>[2x]GSHGQYLLPEAKAQDSDKICVVINLDETLVHSSFKPVNNADFIIPVEIDGV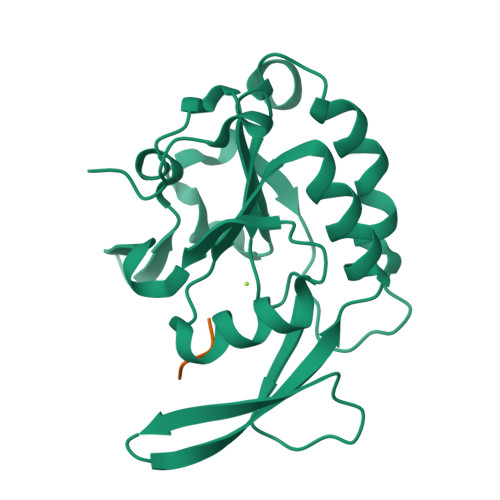VHQVYVLKRPHVDEFLQRMGELFECVLFTASLAKYADPVADLLDKWGAFRARLFRESCVFHRGNYVKDLSRLGRDLRRVLILDNSPASYVFHPDNAVPVASWFDNMSDTELHDLLPFFEQLSRVDDVYSVLRQPRPGS One such enzyme is 2-hydroxyacyl-CoA lyase/synthase (HACL/S), which catalyzes the reversible cleavage of 2-hydroxyacyl-CoA (2hcCoA) into formyl-CoA (fCoA) and an aldehyde or ketone. Originally identified in the mammalian α-oxidation pathway of 3-methyl-branched fatty acids, HACL/S has demonstrated remarkable catalytic reversibility, as it is capable of condensing fCoA with various substrates covering a wide range of aldehydes and ketones with different carbon chain lengths. All the enzymes are tetramers, specifically dimers of dimers (α2), where α2 dimer represents a catalytical unit. The three domains have specific functions: the N-terminal domain binds the pyrimidine of ThDP (PYR), the middle domain has a regulatory function (R) and binds ADP, and the C-terminal domain binds the pyrophosphoryl group (PP) of ThDP.

Structures of both TbHACL/S and ApbHACL/S with and without acyl-CoA indicate that there is no notable difference in main chains and side chains except for the well-ordered C-terminal regions. All structures contain well-defined bound ThDP and ADP. All our HACL/S structures contain bound ADP in the R domain, which assumes the Rossmann fold nucleotide binding unit. ApbHACL/S has stronger activity on C2 (acetaldehyde) compared to C1 (formaldehyde) and C3 (propionaldehyde) substrates, while TbHACL/S discriminates less harshly between substrate chain length.

>[4x]MATITGAQIVARALKQQGVEHMFGIVGIPVIPIAAAAQREGIKFYGFHNEQSASYAAGAVGYLTGRPGVCLAVSGPGMIHGIAGLANAWSNNWPMILIGGANDSYQNGQGAFQEAPQIESARPYVKYAARPDSIARLPFYVEQAVRTTIYGRPGAAYLDLPGDIISGSVEEAEVTYPGRCPEPPRTLAPEENIKAALAALKTAERPLVIVGKGAAYSRAEDEVRKFVETTGLPYLASPMGKGVIPDDHPQSIAAARSFALQNTDLVVLMGARMNWMMHFGQPPRWNEKVRVIQMDISAEEIGTNVPTEVALVGDAKAITAQLNAELEKNPWSYPSETTWWTGLQSKIAANAATVEPMFNDDSVPMGYYRVLRDIRDLIPKDAIISNEGASTMDIGRTVLPNFFARTRLDAATFGTMGVGAGQAIAAASVHPDRKIICVQGDSAFGFGGMEVETAARYGLNITFVIINNNGIGGGPDELDPAHIPPGAYTPQAHYEKMADVYGGKGYFVTTPDQLKPVLEEAMAQPKPAIVNIMISNKSGRKPQEFGWLTR Human manganese superoxide dismutase (MnSOD) is a CPET-based oxidoreductase found in the mitochondrial matrix that reduces ROS levels by eliminating O2•− with the unpaired electrons of the active site metal. The Mn ion is coordinated to inner-sphere residues His26, His74, His163, Asp159, and a single-oxygen species that could be either H2O or –OH (designated WAT1). Trivalent Mn oxidizes O2•− to O2 (k1 = 1.5 nM−1 s−1)8 and the resulting divalent Mn reduces another O2•− molecule to H2O2 (k2 = 1.1 nM−1 s−1). The second sphere of MnSOD harbors five residues (His30, Tyr34, Gln143, Glu162, and Tyr166) and information about their protonation states would be of significant value in deciphering a catalytic mechanism.

To visualize the effect of the electronic state of the metal on the active site protons, all-atom, D-labeled neutron structures were obtained for Mn3+SOD and Mn2+SOD to resolutions of 2.20 and 2.30 Å, respectively. The two data sets collected were from the same crystal treated with appropriate oxidizing and reducing chemicals and the redox conditions were maintained during each data collection. For the oxidized resting state that is described by both chains of the Mn3+SOD neutron structure, the proton bridging His30 and Tyr166 appears to be moving and this suggests the possibility of Tyr166 alternating between an ionized or protonated form and a deprotonated or protonated Nε2(His30). Nδ1(His30) is also observed to be both deprotonated or protonated. An SSHB is seen between WAT2 and an ionized Tyr34 while Gln143 is in the canonical amide form hydrogen bonding to WAT1 as a –OH molecule. Instead, the MnSOD neutron data suggest that the proton donor to WAT1 is internally sourced from Gln143 without the direct involvement of solvent and cannot be Tyr34 due to its observed deprotonation in the Mn3+ state. An ionized tyrosine residue at physiological pH is unusual though is potentially explained by polarization from the pronounced positive charge of the metal. The rates indicate an important role for His30 k1 that may correspond with our observations of its changes in protonation in Mn3+SOD. Starting from the five-coordinate Mn3+ resting state, Mn3+ acquires an electron (in reality from the substrate superoxide) that coincides with Nδ1(His30) acquiring a proton from the nearest solvent molecule (the crystallographic position of WAT2) and Tyr166 gaining partial covalent character from the proton of Nε2(His30) to form a LBHB.

>MKHSLPDLPYDYGALEPHINAQIMQLHHSKHHAAYVNNLNVTEEKYQEALAKGDVTAQIALQPALKFNGGGHINHSIFWTNLSPNGGGEPKGELLEAIKRDFGSFDKFKEKLTAASVGVQGSGWGWLGFNKERGHLQIAACPNQDPLQGTTGLIPLLGIDVWEHAYYLQYKNVRPDYLKAIWNVINWENVTERYMACKK[2x]In this study, we identified four enzymes (two GH183 endo-d-arabinanases, GH172 exo-α-d-arabinofuranosidase, and GH116 exo-β-d-arabinofuranosidase) from Microbacterium arabinogalactanolyticum. These enzymes completely degraded the complex d-arabinan core structure of lipoarabinomannan and arabinogalactan in a concerted manner. Furthermore, through biochemical characterization using synthetic substrates and X-ray crystallography, we elucidated the mechanisms of substrate recognition and anomer-retaining hydrolysis for the α- and β-d-arabinofuranosidic bonds in both endo- and exo-mode reactions. We propose a d-arabinan-degrading pathway for Mi. arabinogalactanolyticum based on its gene cluster and four characterized enzymes.

The crystal structures of EndoMA1 were determined at resolutions of 1.60 and 1.80 Å for the apo and ligand complex forms, respectively. We focused on the complex structure because the apo and complex structures are nearly identical (Cα root mean square deviation (RMSD) < 0.27 Å for all chain pairs). Therefore, we performed experiments of multi-angle static light scattering and refractive index combined with SEC (SEC-MALS/RI) and small-angle X-ray scattering combined with SEC (SEC-SAXS) on EndoMA1 to clarify its quaternary structure in solution. The molar mass estimates of monomeric EndoMA1 calculated by the amino acid sequence and measured by SDS-PAGE were 53,678 Da and 52.4 kDa, respectively, suggesting that EndoMA1 formed a dimer in solution. The experimental SAXS profile (black open circle) and theoretical SAXS profile calculated from the dimeric crystal structure (red line) were in good agreement. In the crystal structure, the active site cleft of the catalytic domain of EndoMA1 adopts the shape of a typical endo-type enzyme (right). A Dali structural search showed that the catalytic domain of EndoMA1 was similar to the hypothetical protein BACOVA_04882, N-acetylgalactosamine deacetylase, and GH43 α-l-Araf-ases. The C-terminal putative CBM domain in EndoMA1 is conserved only in its closest homologs. EndoMA1 and EndoMA2, two new GH family endo-d-arabinanases with signal sequences, depolymerize mycobacterial lipoarabinomannan and arabinogalactan extracellularly.

>[4x]MTTSRTPATVVEKLTGPDAPNNTWGRWDIKATDLGIMWDDGAGHVLTAFGDTFGNSWTGPGGGAPPNGNWRSNVLVRSSDGDLADGMLFDWAAQGPQGVAREIIPSKKINGVEITTIPTTGISVGKRQYLGFMSVKQWGPPGVWDTNFAGIAYSDDGGGTWKVSDTRWENADGHDPFQMQAWVQKGGTIYVFGTQNGRNGPASVAKVPASKLLDKSAFRYWNGTDWSRKESDAVPVMDAPMSEMSVQYDAYSKRFLMMTLSGEDIIMRTATAPEGPWTPAQTVASSTDYPALYGGYFHPWNKDGEIYFTMSQWNPYNVYLMRLRIDRDGNIIDPNLVTDASFERSTTLGDGTNGTWAAKPNSGIDNAPAAGFTGDHRAFVRYNSGWRDIWQDVAVERGAKYRLTGFLRTSVNSDNGFFGARTLDGVPIGEINFHSVGAWTRFTVEFDAGDRDAVQVFGGVWTNSGDIWMQLDDVSLTKVRLEHHHHHH> XFVYSA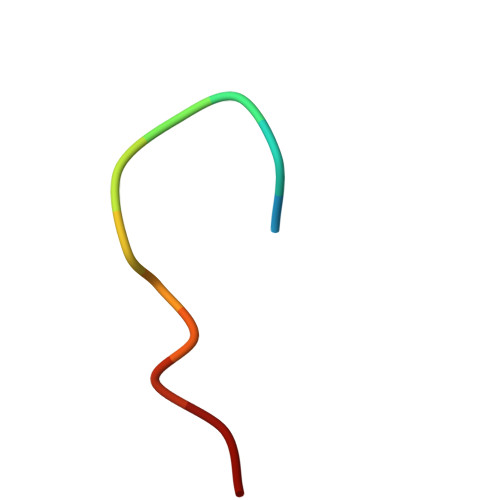VCAAAA>[12x]GSPAEIASFSPRPSLADSK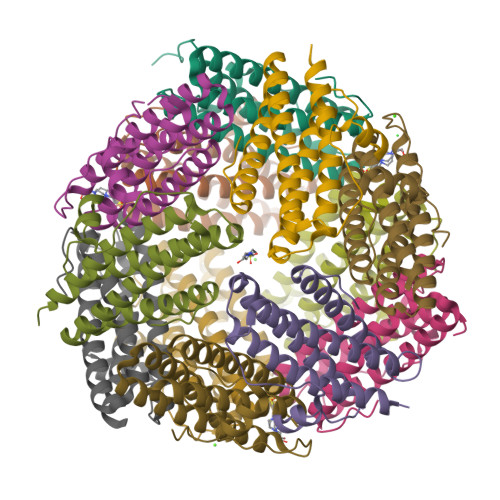AVLNQAVADLSVAHSILHQVHWYMRGRGFMIWHPKMDEYMEEIDGYLAEMSERLITLGGAPFSTLKEFSENSQLKEVLGDYNVTIEEQLARVVEVFRYLAALFQKGFDVSDEEGDSVTNDIFNVAKASIEKHIWMLQAELGQAPKL> MLRRFALTSSVALRLRFERDSGHNTVRYRPIPESMQPKHLEDNFTPFPLPKFDESLEYGPVRLRNIPDIEAAKERRRGSRLAATEVLLQETLQEENQFATSGKGDGNMAIAITERHTEDVTTPAADSRFPSQTMSPCSHEEEMRGYVVSRDYPLIDRLHCTRSIEELVAQFEDRPQIESRVAALADMASTVSFRSDEELLRMFTAISAPFSVDGRGLNFLTVKVSKFGRPYYVPNSLLPAYVNLVDATTIALVREQPWRLSASPALFIQVLQFMALIKVFEPNKWFTFSDHAPSNRADYRHAIGVNHSTAFWGTGEELYDFMVELLRVEDDGRIPTMLDLCTREQMVDLLSGFCGVMPCGKAVGDVFKTITDAFLRRVRNDISGPWSAHDWAIVERMYLVTVLCDAGNNEILQLLLSDTASPRGPDFFAAVSRTKDTPTKKRALCLLQEAIDNASAKADKVTLLGLLESGSEFLLSLVDKGVAHTFATQNLFDYRILNSFLHCSLVADRLRVEQSVITSLIPSSLRDVQVQMLMSNERNALNPLTSSLPGNSGAIATAPKLKRPLMTMLSQLEYLNSIDSVFILHSSLMATSTDQLVSAVRRLPSGKDSLIVTMSCLRALSVKSLTSPSMKERIACARALEIVSYELEKGRAVLLPFSEEILLHDAGAYCDEDLMLWTVAAFLARELPLVKVHTLMHSNCTARTPYRFLKGGHNLLVSSRSLYDKGAPLLSSLHSKELRLVTHNVRLRTPVRDRKCTLQYYNPIRARFVYRRDKPLFDKYHVTARNLAPGFSRGALKHDWRALGVY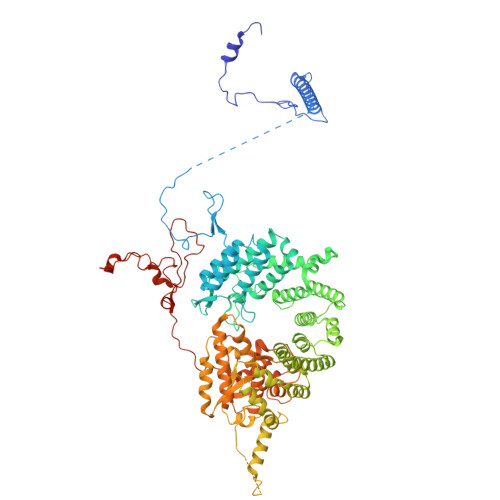TPDHPQVPYHPLQTWMLGETTVEAE(3~{S})-3-[1-[4,5-bis(chloranyl)-1~{H}-benzimidazol-2-yl]-3-methyl-5-oxidanyl-pyrazol-4-yl]-3~{H}-2-benzofuran-1-one | C19 H12 Cl2 N4 O3 | 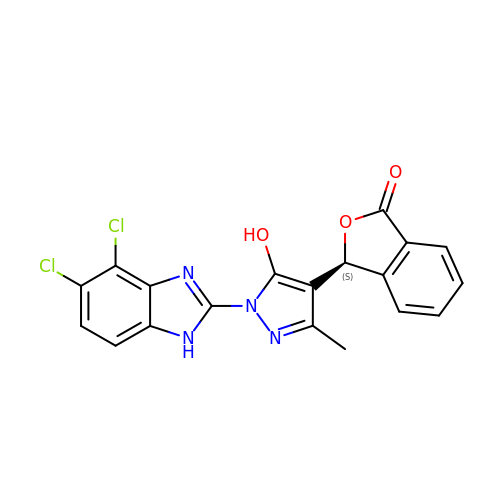VIQXILLOJLATEF-INIZCTEOSA-N>[8x]DDDDDDISDDNIKVDPSLKFENPSLRQAY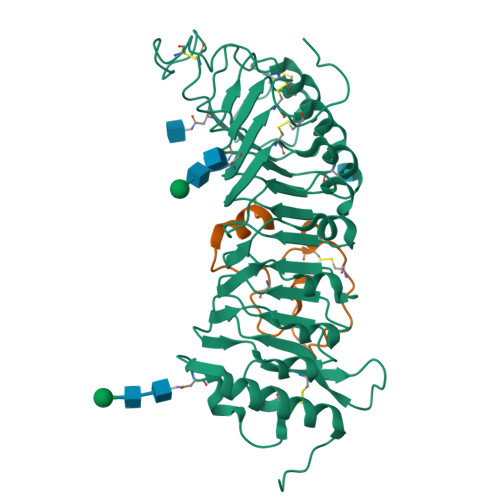IALQSWKQAIFSDPFNFTANWNGSDVCSYNGIFCAPSPSSPKTRVVAGIDLNHADMAGYLPRELGLLTDLALFHLNSNRFCGEVPLTFKHMKLLFELDLSNNRFVGKFPNVVLSLPSLKFLDLRYNEFEGSIPSKLFDKELDAIFLNHNRFMFGIPENMGNSPVSALVLADNDLGGCIPGSIGLMGKTLNEIILSNDNLTGCLPPQIGNLKNVTVFDISFNRLSGPLPSSIGNMKSLEQLNVANNRFTGVIPSSICQLSNLENFTYSSNFFTGDAPRCVALLGDNVVVNGSMNCIDGKEDQRSSKECSSPASRSVDCSKFGCNNFFSPLENL;>MGRRQLARGRRYIGYDALKKNNVPCSRRGRSYYDCKKRRRNNPYRRGCSAITHCYR[8x]>[4x]KL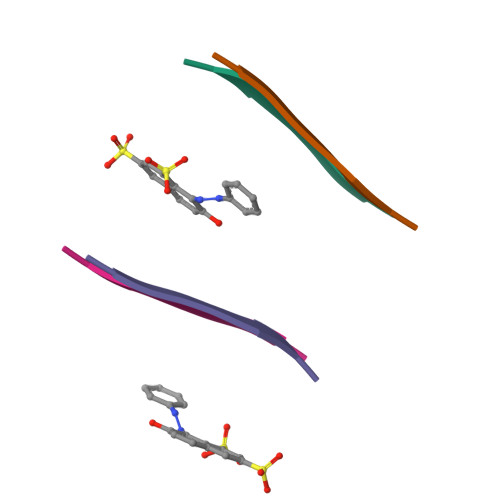VFFA> GUGUGCCCGGCAUGGGUGCAGUCUAUAGGGUGAGAGUCCCGAACUGUGAAGGCAGAAGUAACAGUUAGCCUAACGCAAGGGUGUCCGUGGCGACAUGGAAUCUGAAGGAAGCGGACGGCAAACCUUCGGUCUGAGGAACACGAACUUCAUAUGAGGCUAGGUAUCAAUGGAUGAGUUUGCAUAACAAAACAAAGUCCUUUCUGCCAAAGUUGGUACAGAGUAAAUGAAGCAGAUUGAUGAAGGGAAAGACUGCAUUCUUACCCGGGGAGGUCUGGAAACAGAAGUCAGUAGAAGUCAUAGUACCCUGUUCGCAGGGGAAGGACGGAACAAGUAUGGCGUUCGCGCCUAAGCUUGAACUGCCGUAUACCGAACGGUACGUACGGUAGUGUG;> GGGGUUAU

Group II introns are ubiquitous self-splicing ribozymes and retrotransposable elements evolutionarily and chemically related to the eukaryotic spliceosome, with potential applications as gene-editing tools. The site also harbors a metal-ion cluster formed by two divalent (M1–M2) and two monovalent (K1–K2) ions. In the first step of splicing, depending on whether the intron follows a hydrolytic or a transesterification mechanism, respectively, a water molecule or the 2′-OH group of a bulged adenosine in D6, activated by M2 and by the triple helix, attack the 5′-splice junction of the precursor (5e-I-3e), forming an intron/3′-exon intermediate (I-3e), in which the scissile phosphate (SP) is coordinated by K2. In the second step of splicing, the 5′-exon (5e), activated by M1, performs a nucleophilic attack on the 3′-splice junction, releasing ligated exons (5e-3e) and a linear or lariat form of the excised intron.

After incorporating the resulting triple base mutations (C289A/C358A/G385U, aka the A-mutant; C289G/C358G/G385C, aka the G-mutant; and C289U/C358U/G385A, aka the U-mutant), we monitored effects on splicing kinetics. First, we determined crystal structures of the G and U mutants in the presence of potassium and magnesium at 3.4 and 3.6 Å resolution, respectively. Importantly, both mutant structures adopt the triple-helical configuration that corresponds with that of the wild-type intron structure. The Fo − Fc simulated-annealing electron density omit maps calculated by omitting the J2/3 residues and the catalytic metal cluster reveal strong electron density signal for the triple helix conformer, as in wild type (total peak height for the nucleobase of G288 = 8.9 σ and 6.7 σ for the G and U mutants, respectively; maximum peak height for the metals = 9.5 σ and 6.6 σ for the G and U mutants, respectively; Fig. 2b). Moreover, the Fo − Fc maps calculated by omitting the first intron nucleotide (G1) show that the 5′-splice junction has undergone cleavage in both mutants during the crystallization process. G1 is unresolved in the structure of the U-mutant. d Superposition of the active sites of the structures depicted in (a). e Secondary structure of the wild-type O. iheyensis group II intron with catalytic site elements highlighted by red boxes and nucleotides not present in the crystal structures in gray. We found that the A-mutant—which can be protonated at position 358—splices at rates comparable to wild type, whereas the G and U mutants—which cannot be protonated at position 358—have splicing defects. Remarkably, splicing defects of the A-mutant are minimal (approximately twofold) and crucially, they do not lead to accumulation of an I-3e intermediate, suggesting that the defects of the G and U mutants predominantly derive from their inability to become protonated at position 358.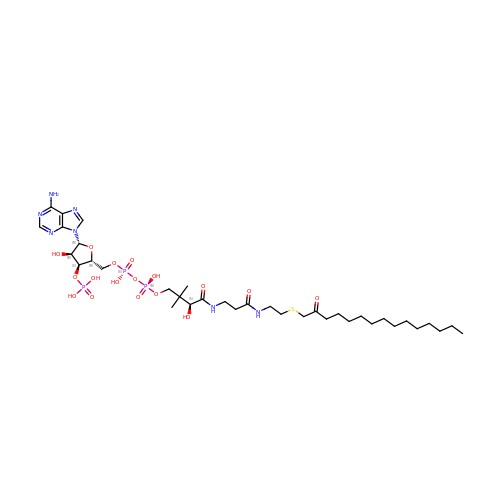S-(2-OXO)PENTADECYLCOA | C36 H64 N7 O17 P3 S | JKWHUJMJVNMKEF-SXKLBCNJSA-N naphthalene-1,2,4,5,7-pentol | C10 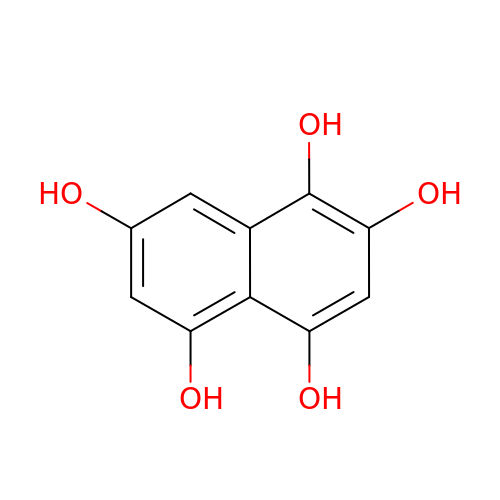H8 O5 | IISYZEMBGRNYTH-UHFFFAOYSA-N> MHHHHHHGSPMTMDEKYVNSIWDLLKNAIQEIQRKNNSGLSFEELYRNAYTMVLHKHGEKLYTGLRE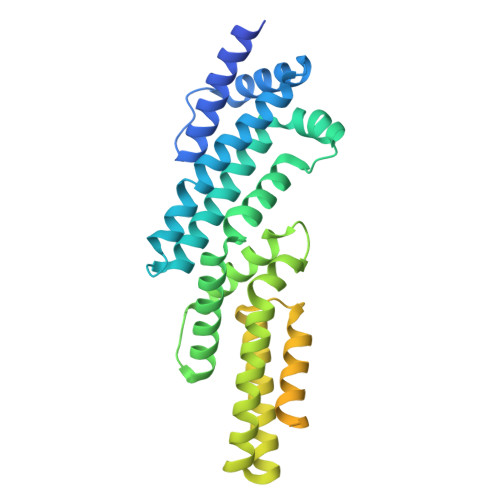VVTEHLINKVREDVLNSLNNNFLQTLNQAWNDHQTAMVMIRDILMYMDRVYVQQNNVENVYNLGLIIFRDQVVRYGCIRDHLRQTLLDMIARERKGEVVDRGAIRNACQMLMILGLEGRSVYEEDFEAPFLEMSAEFFQMESQKFLAENSASVYIKKVEARINEEIERVMHCLDKSTEEPIVKVVERELISKHMKTIVEMENSGLVHMLKNGKTEDLGCMYKLFSRVPNGLKTMCECMSSYLREQGKALVSEEGEGKNPVDYRQGLDDLKSRFDRFLLESFNNDRLFKQTIAGDFEYFLNLNSRSPEYL> GSHMTAYTAERQPERDITPVNDETMQEINTLLIALDKTWDDDLLPLCSQIFRRDIRASSE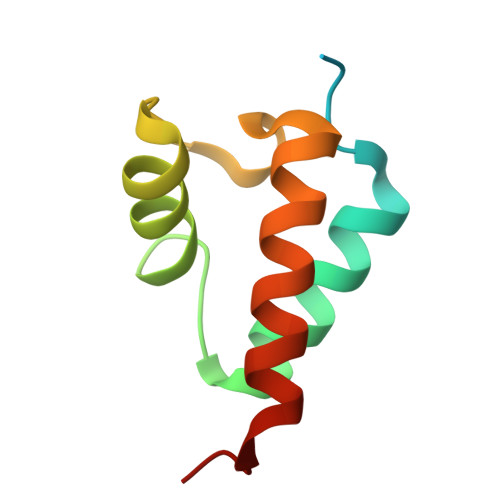LTQAEAVKALGFLKQKAAEQKVAA> MATTADFKNGLVLKNEGKLQQIIEFQHVKPGKGPAFVRTKLKDVVTGKTIDKTWNAGVKVETATVDR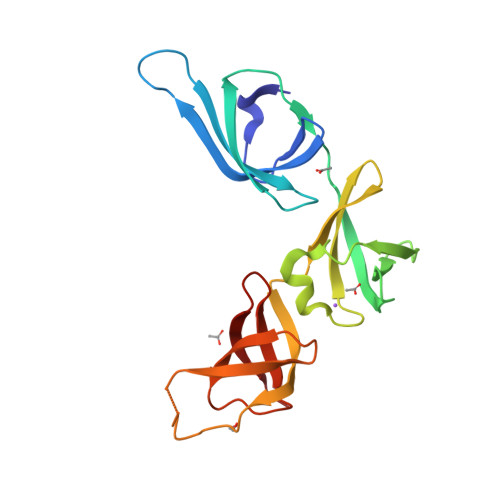RDVTYLYNDGTSFIVMDDKTFEQYELSPDAFGDAGRFLLENMRVQVSFHEGEALFGELPVSVDLRVEHTDPGLQGDRSTGGTKPATLETGAEIQVPLFIETGNVLKVDTRDGSYLSRVNN>MKIATYNVRVDTEYDQDWQWSFRKEAVCQLINFHDWSLCCIQEVRPNQVRDLKAYT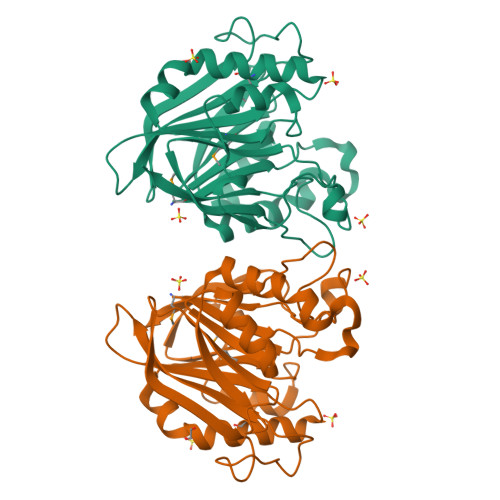TFTCLSAEREGDGQGEGLAILYNEQKVQAIDTGYFWLSETPQQPSIHPEAGCPRIALWGLFKETTQNTPFLVINVHLDHISAHARLAGMTVILEELHDKIAQYPTLLMGDFNAESGEEVHQLVQKKFQDSKNLATHYGPRGTFQNFTYTKPWAELEEIDYIYVKGWQVQQTASLTDSIDGRFPSDHFPLEAEVAGENLYFQ[6x]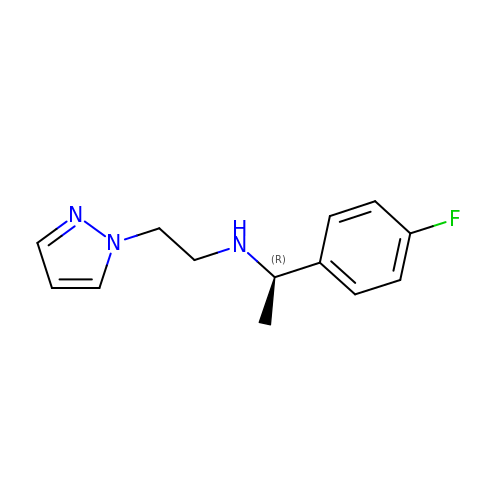(1R)-1-(4-fluorophenyl)-N-[2-(1H-pyrazol-1-yl)ethyl]ethan-1-amine | C13 H16 F N3 | GDFKNYCJQSHPRK-LLVKDONJSA-N>[2x]MSAIENFDAHTPMMQQYLRLKAQHPEILLFYRMGDFYELFYDDAKRASQLLDISLTKRGASAGEPIPMAGIPYHAVENYLAKLVNQGESVAICEQIGDPATSKGPVERKVVRIVTPGTISDEALLQERQDNLLAAIWQDSKGFGYATLDISSGRFRLSEPADRETMAAELQRTNPAELLYAEDFAEMSLIEGRRGLRRRPLWEFEIDTARQQLNLQFGTRDLVGFGVENAPRGLCAAGCLLQYAKDTQRTTLPHIRSITMEREQDSIIMDAATRRNLEITQNLAGGAENTLASVLDCTVTPMGSRMLKRWLHMPVRDTRVLLERQQTIGALQDFTAGLQPVLRQVGDLERILARLALRTARPRDLARMRHAF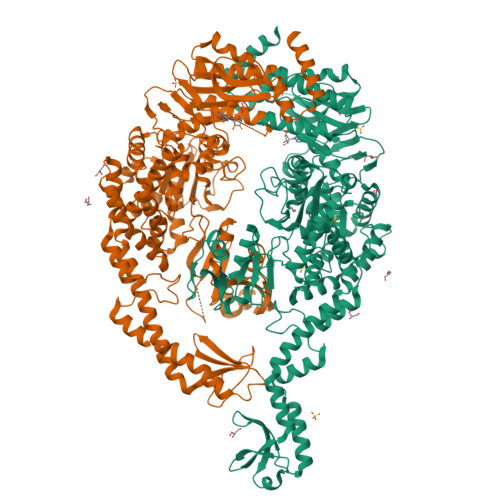QQLPELRAQLETVDSAPVQALREKMGEFAELRDLLERAIIDTPPVLVRDGGVIASGYNEELDEWRALADGATDYLERLEVRERERTGLDTLKVGFNAVHGYYIQISRGQSHLAPINYMRRQTLKNAERYIIPELKEYEDKVLTSKGKALALEKQLYEELFDLLLPHLEALQQSASALAELDVLVNLAERAYTLNYTCPTFIDKPGIRITEGRHPVVEQVLNEPFIANPLNLSPQRRMLIITGPNMGGKSTYMRQTALIALMAYIGSYVPAQKVEIGPIDRIFTRVGAADDLASGRSTFMVEMTETANILHNATEYSLVLMDEIGRGTSTYDGLSLAWACAENLANKIKALTLFATHYFELTQLPEKMEGVANVHLDALEHGDTIAFMHSVQDGAASKSYGLAVAALAGVPKEVIKRARQKLRELESISPNAAATQVDGTQMSLLSVPEETSPAVEALENLDPDSLTERQALEWIYRLKSLV Functional ParMRC plasmid segregation systems comprise an actin-like polymerizing motor (ParM), a centromere-like specific DNA sequence (parC), and an adaptor protein (ParR), which attaches a plasmid, via the parC, to each end of the growing ParM filament or filament bundle. Thus, the force generated from ParM polymerization is harnessed for plasmid segregation. Here we investigated the ParMRC cassette from pCBH, a 257 kb plasmid that carries the botulinum neurotoxin type B. This ParMRC cassette is also found on other C. botulinum plasmids, such as pCLK (267 kb) and pRSJ2_3 (245 kb), which encode neurotoxin types A and F, respectively. Despite the similarities to actin, pCBH ParM is a genuine ParM, since it has a closed β-barrel, a feature that is missing from actin and MreB structures.

Using the E. coli R1 ParM cryoEM protofilament structure as a template, we designed a quadruple mutant of pCBH ParM that was predicted to prevent polymerization. Mutations to subdomain 2 (F42D, I46D) and subdomain 3 (S298D and R299D) were expected to disrupt intra-protofilament subunit contacts, with subdomains 1 and 4. X-ray crystallography studies on the quadruple mutant, using the cryoEM density map as a molecular replacement model, led to the 3.25 Å structure of the monomer (G-ParM), which was subsequently used as a guide to construct the filament protomer structure in the cryoEM density (F-ParM). Two of the mutation sites (Phe42 and Arg299), from the quadruple mutant, were observed to participate in intra-protofilament subunit contacts. This accounts for the success of the quadruple mutant in the preventing filament formation and allowing for monomer crystallization. The major difference between the monomer and filament protomers was the folding of a disordered region into a helix in F-ParM (F helix). This region is equivalent to the DNase I binding loop in actin, which is generally disordered in G-actin and becomes ordered to form a defined extended loop in F-actin. The nucleotide-binding site in the pCBH G-ParM and F-ParM structures contain ADP and the magnesium ion is coordinated by Asp9, Asp195, and Gln168 equivalent to Asp11, Asp154, and Gln137 in actin, suggesting a common mechanism of ATP hydrolysis in which Gln168 (Gln137) directs the hydrolytic water towards the ATP γ-phosphate for nucleophilic attack. Actin residue His161, which has also been proposed to be the catalytic base in ATP hydrolysis, is not conserved in the pCBH ParM structure and has the opposite charge, Asp202, indicating that the conserved glutamine may represent the evolutionary conserved residue important for hydrolysis.

>[3x]GPMNKYTIAIDLGYGQIKGINQDNKRVIFPSIISSGKDRSLDTDFNSDDNIVDNIHVKILDEYFNEKEYFVGELAKRQPSNSSFINRDNKINSEENKVLLATALGLLIPNDLPNDTKIHIVTGLPLEHFIKQKQALNDMLKDFEHTIKFVDHNFSRNIKFEESNITLFPQGAGAIFSKINNDISSLLIKETFIGLIDVGFKTTDIVVFRINKDKEPVFEQEMSATLDGLGMINIYNTMDKAFTDNSRDGSKLNTEQLMLLCEEGKIFFKGDYIDLKKDLIKARKTLSTNIINKADGLWGDDKNSFNSIMIAGGGGKVLYNHLKLIEPNMCQLIDNPEFANAIGYLEFGKQFK>[2x]GSMSSPYILVLYYSRHGATAEMARQIARGVEQGGFEARVRTVPAVSTECEAVAPDIPAEGALYATLEDLKNCAGLALGSPTRFGNMASPLKY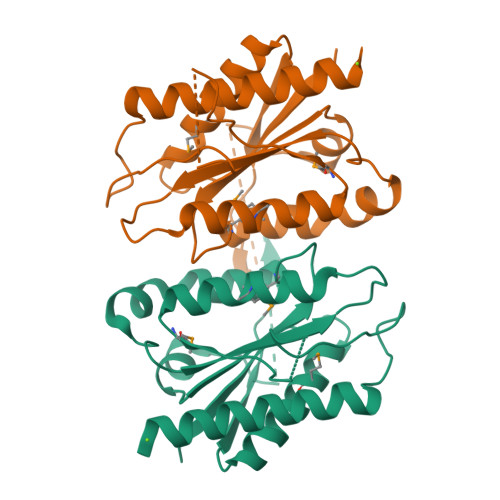FLDGTSSLWLTGSLVGKPAAVFTSTASLHGGQETTQLSMLLPLLHHGMLVLGIPYSEPALLETRGGGTPYGASHFAGADGKRSLDEHELTLCRALGKRLAETAGKLGS> HYNG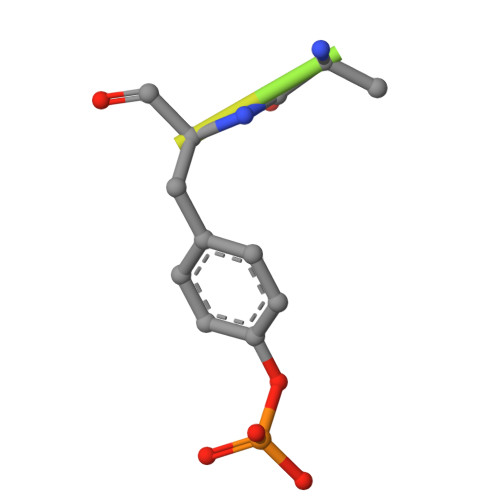EAYEDDEHH> ASINYDQNYQTGGQVSYSPSNTGFSVNWNTQDDFVVGVGWTTGSSAPINFGGSFSVNSGTGLL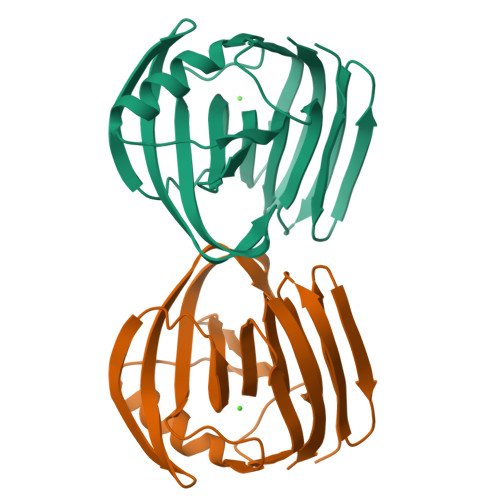SVYGWSTNPLVEYYIMEDNHNYPAQGTVKGTVTSDGATYTIWENTRVNEPSIQGTATFNQYISVRNSPRTSGTVTVQNHFNAWASLGLHLGQMNYQVVAVEGWGGSGSASQSVSN> RGSHHHHHHTDPALRAITHISPLGSMDMLSQLEVDMLKRTASSDLYQLFRNCSLAVLNSGSLTDNSKELLSRFENFDINVLRRERGVKLELINPPEEAFVDGRIIRALQANLFAVLRDILFVYGQIHNTVRFPNLNLDNSVHITNLVFSILRNARALHVGEAPNMVVCWGGHSINENEYLYARRVGNQLGLRELNICTGCGPGAMEAPMKGAAVGHAQQRYKDSRFIGMTEPSIIAAEPPNPLVNELIIMPDIEKRLEAFVRIAHGIIIFPGGVGTAEELLYLLGILMNPANKDQVLPLILTGPKESADYFRVLDEFVVHTLGENARRHYRIIIDDAAEVARQMKKSMPLVKE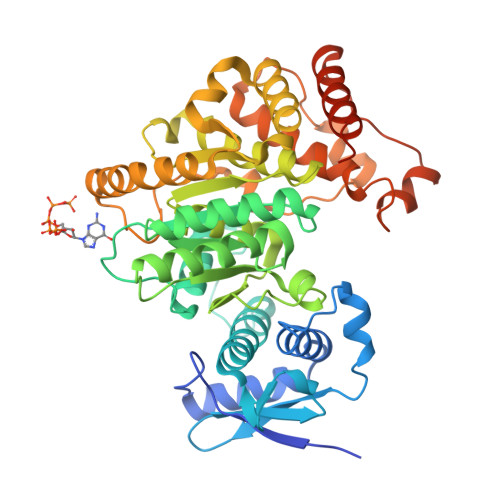NRRDTGDAYSFNWSMRIAPDLQMPFEPSHENMANLKLYPDQPVEVLAADLRRAFSGIVAGNVKEVGIRAIEEFGPYKINGDKEIMRRMDDLLQGFVAQHRMKLPGSAYIPCYEICTGLCGR>[2x]MTHPIIHDLENRYTSKKYDPSKKVSQEDLAVLLEALRLSASSINSQPWKFIVIESDAAKQRMHDSFANM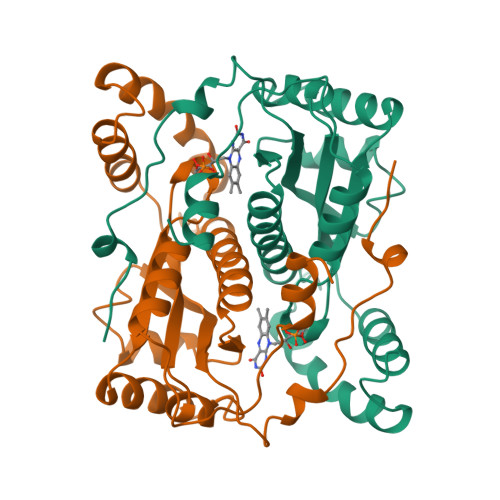HQFNQPHIKACSHVILFANKLSYTRDDYDVVLSKAVADKRITEEQKEAAFASFKFVELNCDENGEHKAWTKPQAYLALGNALHTLARLNIDSTTMEGIDPELLSEIFADELKGYECHVALAIGYHHPSEDYNASLPKSRKAFEDVITIL>MPETEEISKGLEDVNIKWTRLTTIDGNKGILRYGGYSVEDIIASGAQDEEIQYLFLYGNLPTEQELRKYKETVQKGYKIPDFVINAIRQLPRESDAVAMQMAAVAAMAASETKFKWNKDTDRDVAAEMIGRMSAITVNVYRHIMNMPAELPKPSDSYAESFLNAAFGRKATKEEIDAMNTALILYTDHEVPASTTAGLVAVSTLSDMYSGITAALAALKGPLHGGAAEAAIAQFDEIKDPAMVEKWFNDNIINGKKRL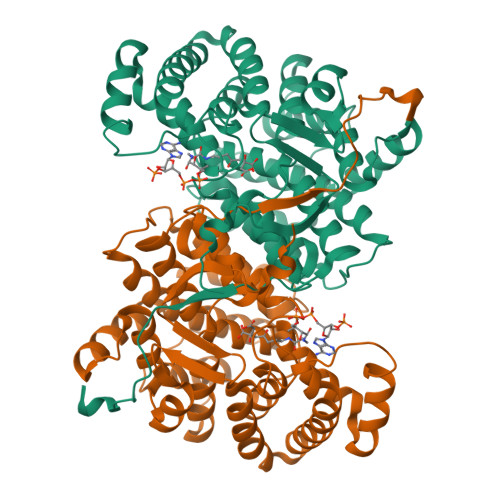MGFGHRVYKTYDPRAKIFKGIAEKLSSKKPEVHKVYEIATKLEDFGIKAFGSKGIYPNTDYFSGIVYMSIGFPLRNNIYTALFALSRVTGWQAHFIEYVEEQQRLIRPRAVYVGPAERKYVPIAERK[4x]>[2x]GSHMDGLLNPRESSKFIAENSRDVFIDSGG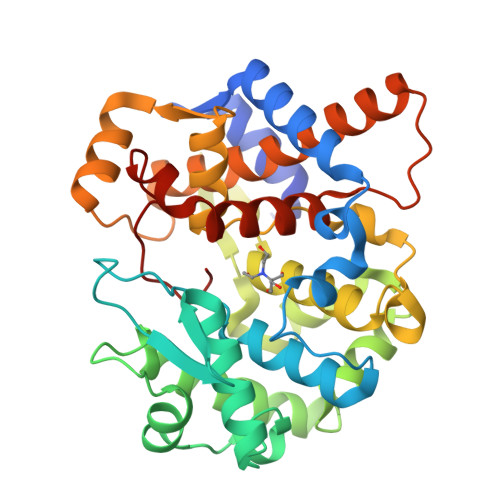VRRVAELLLAKAAGPELRVEGWKALHELNPRAADEAAVNWVFVTDTLNFSFWSEQDEHKCVVRYRGKTYSGYWSLCAAVNRALDEGIPITSASYYATVTLDQVRNILRSDTDVSMPLVEERHRILNETGKILLEKFGGSFLNCVRESENSAQKLMHLVVESFPSYRDVTLFEGKRVSFYKRAQILVADTWSVLEGKGDGCFKDISSITMFADYRLPQVLAHLGALKYSDDLLKKLLKGEMLSYGDRQEVEIRGCSLWCVELIRDCLLELIEQKGEKPNGEINSILLDYYLWDYAHDHREDMKGIPFHRIRCIYY>[2x]MLFRAVLLCAALGLSQAANHHHHHHPCCSNPCQNRGECMSTGFDQYKCDCTRTGFYGENCTTPEFLTRIKLLLKPTPNTVHYILTHFKGVWNIVNNIPFLRSLIMKYVLTSRSYLIDSPPTYNVHYGYKSWEAFSNLSYYTRALPPVADDCPTPMGVKGNKELPDSKEVLEKVLLRREFIPDPQGSNMMFAFFAQHFTHQFFKTDHKRGPGFTRGLGHGVDLNHIYGETLDRQHKLRLFKDGKLKYQVIGGEVYPPTVKDTQVEMIYPPHIPENLQFAVGQEVFGLVPGLMMYATIWLREHNRVCDILKQEHPEWGDEQLFQTSRLILIGETIKIVIEDYVQHLSG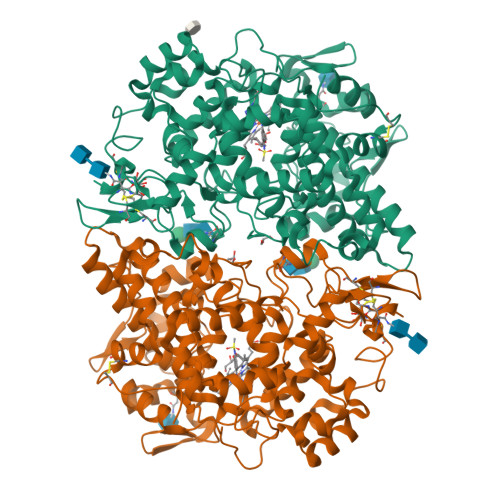YHFKLKFDPELLFNQQFQYQNRIASEFNTLYHWHPLLPDTFNIEDQEYSFKQFLYNNSILLEHGLTQFVESFTRQIAGRVAGGRNVPIAVQAVAKASIDQSREMKYQSLNEYRKRFSLKPYTSFEELTGEKEMAAELKALYSDIDVMELYPALLVEKPRPDAIFGETMVELGAPFSLKGLMGNPICSPQYWKPSTFGGEVGFKIINTASIQSLICNNVKGCPFTSFNVQDPQPTKTATIAASASHSRLDDINPTVLIKRRSTEL> PAKDVQICPIAVDTTVFRSRTWDRLKFEIEYGLQRGTTANSYLISADKIALFDPPGESFTDNFVGTLIQRLDLNSLDYVILGHVNANRAHTLKLLLSLAPQATIICSNPAAQNLEKLLADAEVNNPIQVMKGNDHLDLGRGHELTFIPTPSPRYPGQLCTYDPRTEILFTDKLFGAHVCGDQVFDEGWTIYQEDRRYYFDCLLAPAAAQVSAALNKLEAYPAQTYAPSHGPLVRYGLRELTRNYQQWLSEQQAQALNVALIYASAYGNT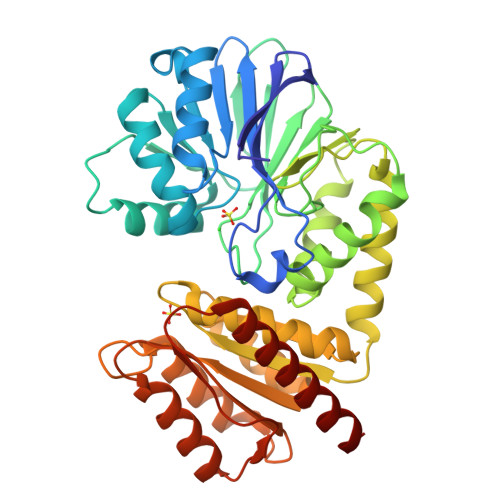STLAQAIARGITKAGVAVTAINAETSNAEEIKEAIGKSAGFIFGSPTLGGHAPTPIQTALGITLANASKTQLCGVFGSFGWSGEAIDMLENKFRDAGFSFGFDTIRVKFKPTDQTLKMCEEAGTDFAQALKKAE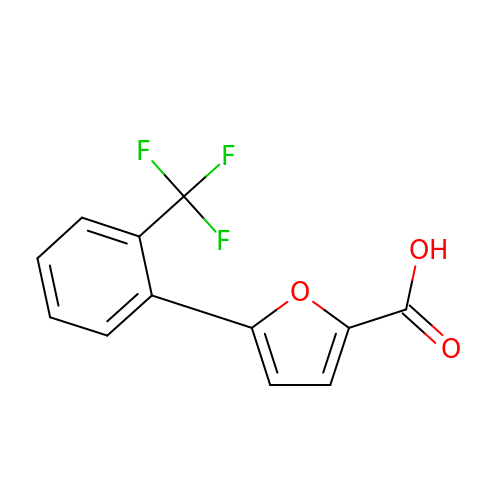5-[2-(TRIFLUOROMETHYL)PHENYL]-2-FUROIC ACID | C12 H7 F3 O3 | IJPNRBZMRINMMR-UHFFFAOYSA-N> MGKLDDFDLDVKVKADTTKVG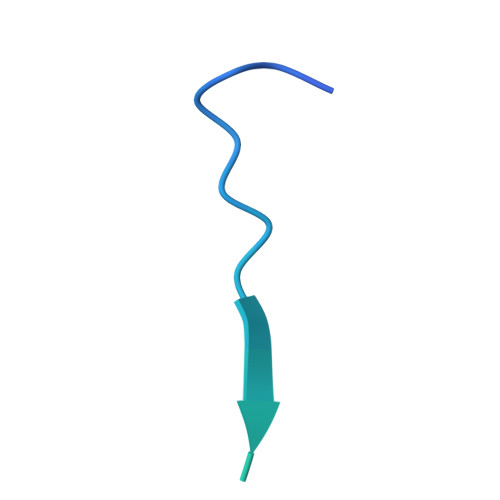PAITSKSLCTPGCITGVLMCITQNSCVSCKSCIKC> VGSLNCIVAVSQNMGIGKNGDLPWPPLRNERRYFERMTTTSSVEGKQNLVIMGKKTWFSIPEKNRPLKGRINLVLSRELKEPPQGAHFLSRSLDDALKLTEQPELANKVDMVWIVGGSSVYKEAMNHPGHLKLFVTRIMQDFESDTFFPEIDLEKYKLLPEYPGVLSDVQE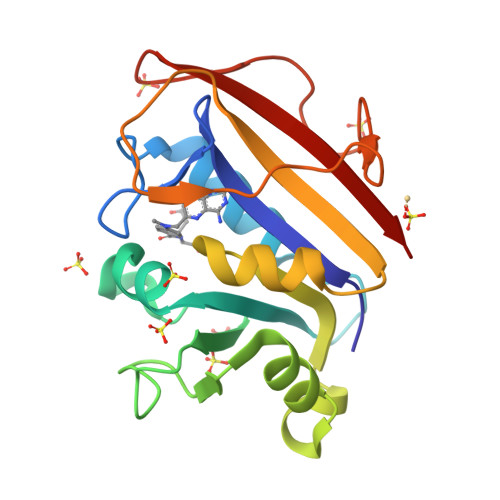EKGIKYKFEVYEKND> QVVASNETLYQVVKEVKPGGLVQIADGTYKDVQLIVSNSGKSGLPITIKALNPGKVFFTGDAKVELRGEHLILEGIWFKDGNRAIQAWKSHGPGLVAIYGSYNRITACVFDCFDEANSAYITTSLTEDGKVPQHCRIDHCSFTDKITFDQVINLNNTARAIKDGSVGGPAMYHRVDHCFFSNPQKPGNAGGGIRIGYYRN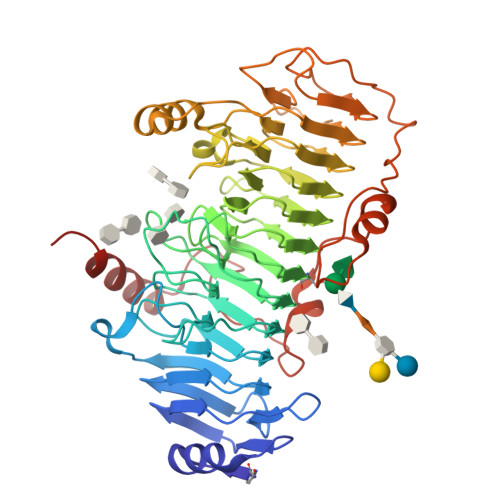DIGRCLVDSNLFMRQDSEAEIITSKSQENVYYGNTYLNCQGTMNFRHGDHQVAINNFYIGNDQRFGYGGMFVWGSRHVIACNYFELSETIKSRGNAALYLNPGAMASEHALAFDMLIANNAFINVNGYAIHFNPLDERRKEYCAANRLKFETPHQLMLKGNLFFKDKPYVYPFFKDDYFIAGKNSWTGNVALGVEKGIPVNISANRSAYKPVKIKDIQPIEGIALDLNALISKGITGKPLSWDEVRPYWLKEMPGTYALTARLSADRAAKFKAVIKRNKEH> IPVIEPLFTKVTEDIPGAEGPVFDKNGDFYIVAPEVEVNGKPAGEILRIDLKTGKKTVICKPEVNGYGGIPAGCQCDRDANQLFVADMRLGLLVVQTDGTFEEIAKKDSEGRRMQGCNDCAFDYEGNLWITAPAGE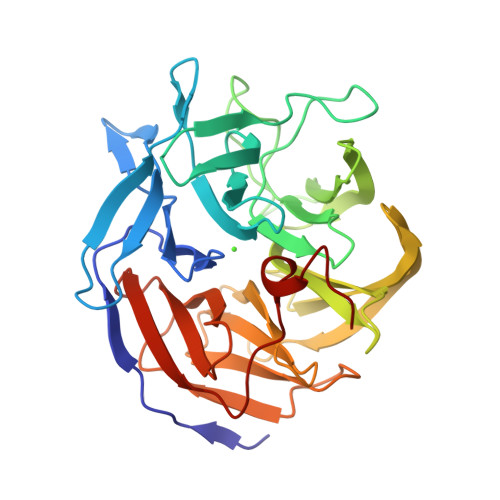VAPADYTRSMQEKFGSIYCFTTDGQMIQVDTAFQFPNGIAVRHMNDGRPYQLIVAETPTKKLWSYDIKGPAKIENKKVWGHIPGTHEGGADGMSFDEDNNLLVANWGSSHIEVFGPDGGQPKMRIRCPFEKPSNLHFKPQTKTIFVTEHENNAVWKFEWQRNGKKQYCETLKFGIF>SRGKGNFSACTHSFGGTRDHDVVEEFIGNIETYKDVEGISDENALKGISLLFYGMASTWWQGVRKEATTWKEAIALIREHFSPTKPAYQIYMEFFQNKQDDHDPIDTFVIQKRALLAQLPSGRHDEETELDLLFGLLNIKYR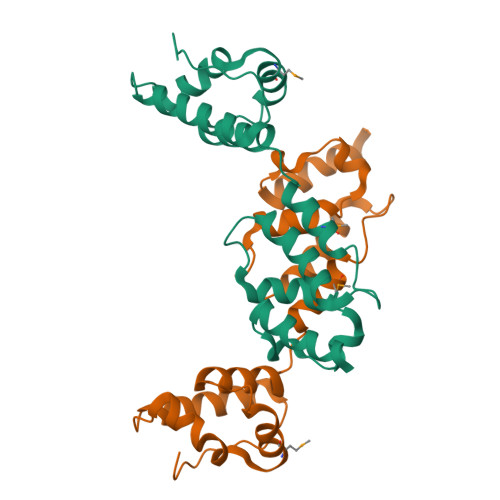KHISRHSVHTFKDLLEQGRIIEHNNPLE[2x]>[2x]MHHHHHHANASETNVGPMAPRVCVVGSVNMDLTFVVDALPRPGETVLAASLTRTPGGKGANQAVAAARAGAQVQFSGAFGDDPAAAQLRAHLRANAVGLDRTVTVPGPSGTAIIVVDASA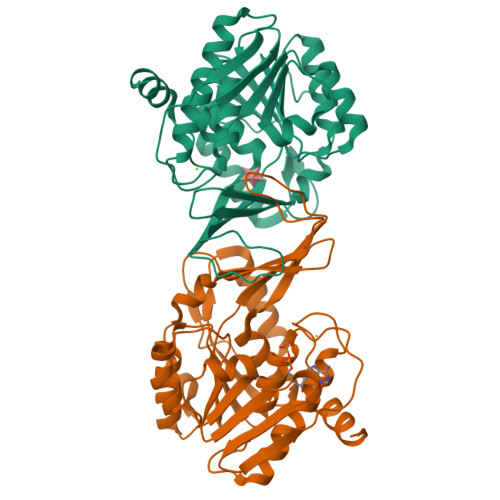ENTVLVAPGANAHLTPVPSAVANCDVLLTQLEIPVATALAAARAAQSADAVVMVNASPAGQDRSSLQDLAAIADVVIANEHEANDWPSPPTHFVITLGVRGARYVGADGVFEVPAPTVTPVDTAGAGDVFAGVLAANWPRNPGSPAERLRALRRACAAGALATLVSGVGDCAPAAAAIDAALRANRHNGS>[6x]MAKKTSSKGKLPPGPRPLPLLGNLLQMDRRGLLKSFLRFREKYGDVFTVHLGPRPVVMLCGVEAIREALVDKAEAFSGRGKIAMVDPFFRGYGVIFANGNRWKVLRRFSVTTMRDFGMGKRSVEERIQEEAQCLIEELRKSKGALMDPTFLFQSITANIICSIVFGKRFHYQDQEFLKMLNLFYQTFSLISSVFGQLFELFSGFL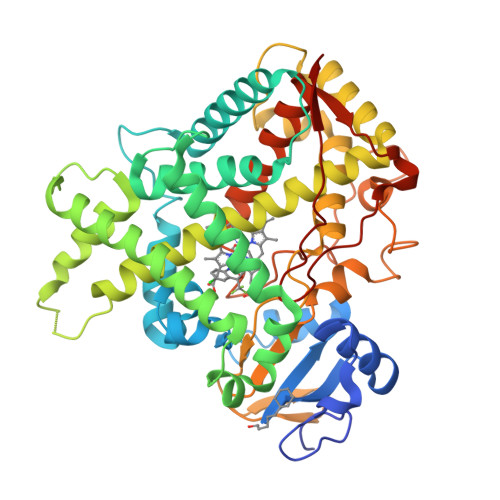KHFPGAHRQVYKNLQEINAYIGHSVEKHRETLDPSAPRDLIDTYLLHMEKEKSNAHSEFSHQNLNLNTLSLFFAGTETTSTTLRYGFLLMLKYPHVAERVYREIEQVIGPHRPPELHDRAKMPYTEAVIYEIQRFSDLLPMGVPHIVTQHTSFRGYIIPKDTEVFLILSTALHDPHYFEKPDAFNPDHFLDANGALKKTEAFIPFSLGKRICLGEGIARAELFLFFTTILQNFSMASPVAPEDIDLTPQECGVGKIPPTYQIRFLPRHHHH> GDPIADMIDQTVNNQVNRSLTALQVLPTAANTEASSHRLGTGVVPALQAAETGASSNASDKNLIETRCVLNHHSTQETAIGNFFSRAGLVSIITMPTTDTQNTDGYVNWDIDLMGYAQLRRKCELFTYMRFDAEFTFVVAKPNGVLVPQLLQYMYVPPGAPKPTSRDSFAWQTATNPSVFVKMTDPPAQVSVPFMSPASAYQWFYDGYPTFGEHLQANDLDYGQCPNNMMGTFSIRTVGTEKSPHSITLRVYMRIKHVRAWIPRPLRNQPYLFKTNPNYKGNDIKCTSTSRDKITTL;> SPSAEACGYSDRVAQLTIGNSTIT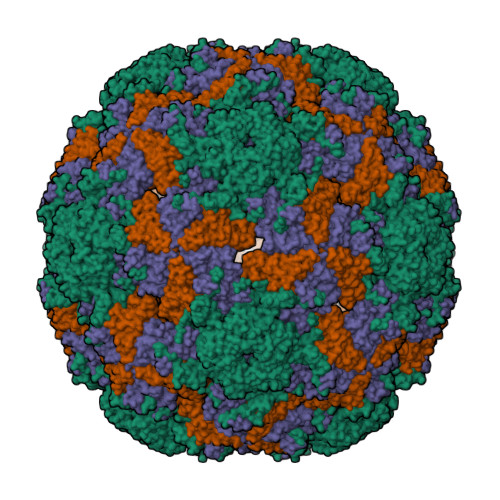TQEAANIVIAYGEWPEYCPDTDATAVDKPTRPDVSVNRFFTLDTKSWAKDSKGWYWKFPDVLTEVGVFGQNAQFHYLYRSGFCVHVQCNASKFHQGALLVAVLPEYVLGTIAGGTGNENSHPPYATTQPGQVGAVLTHPYVLDAGIPLSQLTVCPHQWINLRTNNCATIIVPYMNTVPFDSALNHCNFGLLVIPVVPLDFNAGATSEIPITVTIAPMCAEFAGLRQAVKQ;> GIPTELKPGTNQFLTTDDGVSAPILPGFHPTPPIHIPGEVHNLLEICRVETILEVNNLKTNETTPMQRLCFPVSVQSKTGELCAAFRADPGRDGPWQSTILGQLCRYYTQWSGSLEVTFMFAGSFMATGKMLIAYTPPGGNVPADRITAMLGTHVIWDFGLQSSVTLVVPWISNTHYRAHARAGYFDYYTTGIITIWYQTNYVVPIGAPTTAYIVALAAAQDNFTMKLCKDTEDIEQTANIQ>ATVSAEIPYQIFRDFAENKGQFTPGTTNISIYDKQGNLVGKLDKAPMADFSSATITTGSLPPGDHTLYSPQYVVTAKHVSGSDTMSFGYAKNTYTAVGTNNNSGLDIKTRRLSKLVTEVAPAEVSDIGAVSGAYQAGGRFTEFYRLGGGMQYVKDKNGNRTQVYTNGGFLVGGTVSALNSYNNGQMITAQTGDIFNPANGPLANYLNMGDSGS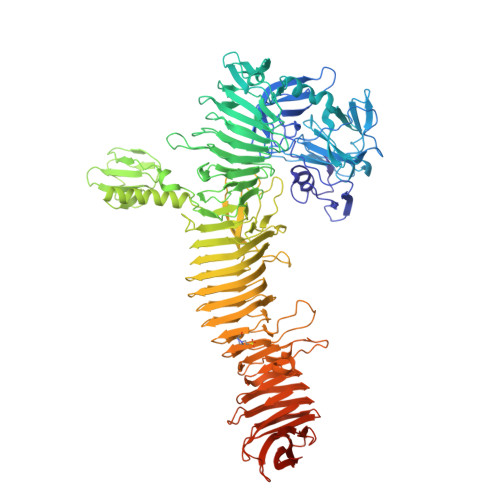PLFAYDSLQKKWVLIGVLSSGTNYGNNWVVTTQDFLGQQPQNDFDKTIAYTSGEGVLQWKYDAANGTGTLTQGNTTWDMHGKKGNDLNAGKNLLFTGNNGEVVLQNSVNQGAGYLQFAGDYRVSALNGQTWMGGGIITDKGTHVLWQVNGVAGDNLHKTGEGTLTVNGTGVNAGGLKVGDGTVILNQQADADGKVQAFSSVGIASGRPTVVLSDSQQVNPDNISWGYRGGRLELNGNNLTFTRLQAADYGAIITNNSEKKSTVTLDLQTLKASDINVPVNTVSIFGGRGAPGDLYYDSSTKQYFILKASSYSPFFSDLNNSSVWQNVGKDRNKAIDTVKQQKIEASSQPYMYHGQLNGNMDVNIPQLSGKDVLALDGSVNLPEGSITKKSGTLIFQGHPVIHAGTTTSSSQSDWETRQFTLEKLKLDAATFHLSRNGKMQGDINATNGSTVILGSSRVFTDRSDGTGNAVSSVEGSATATTVGDQSDYSGNVTLENKSSLQIMERFTGGIEAYDSTVSVTSQNAVFDRVGSFVNSSLTLGKGAKLTAQSGIFSTGAVDVKENASLTLTGMPSAQKQGYYSPVISTTEGINLEDNASFSVKNMGYLSSDIHAGTTAATINLGDSDADAGKTDSPLFSSLMKGYNAVLRGSITGAQSTVNMINALWYSDGKSEAGALKAKGSRIELGDGKHFATLQVKELSADNTTFLMHTNNSRADQLNVTDKLSGSNNSVLVDFLNKPASEMSVTLITAPKGSDEKTFTAGTQQIGFSNVTPVISTEKTDDATKWVLTGYQTTADAGASKAAKDFMASGYKSFLTEVNNL[2x]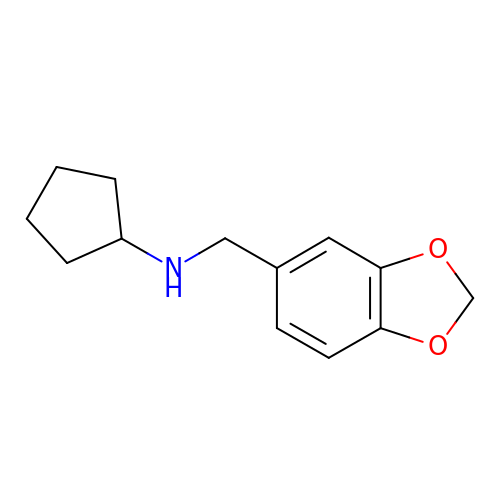N-(1,3-benzodioxol-5-ylmethyl)cyclopentanamine | C13 H17 N O2 | LOYZMUZNAPZSOX-UHFFFAOYSA-N>[2x]MAIEIVERSNYMGNPWTEYMAKYDIEEVHGSGIRVDLGEDAEVAGTQYRLPSGKCPVFGKGIIIENSNTAFLTPVATGNQYLKDGGFAFPPTEPLMSPMTLDEMRHFYKDNKYVKNLDELTLCSRHAGNMIPDNDKNSNYKYPAVYDDKDKKCHILYIAAQENNGPRYCNKDESKRNSMFCFRPAKDISFQNY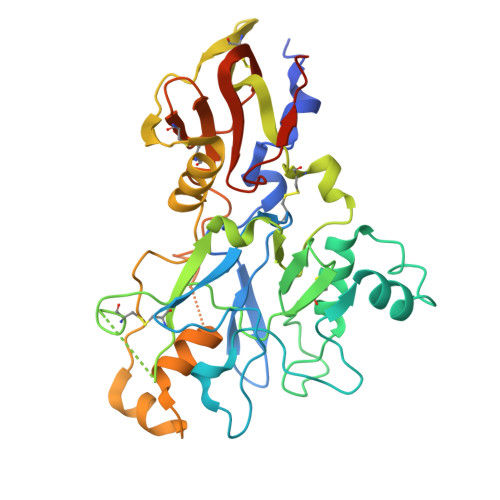AYLSKNVVDNWEKVCPRKNLQNAKFGLWVDGNCEDIPHVNEFPAIDLFECNKLVFELSASDQPKQYEQHLTDYEKIKEGFKNKNAAMIKSAFLPTGAFKADRYKSHGKGYNWGNYNTETQKCEIFNVKPTCLINNAAYIATTALSHPIEVENNFPAAAHHHHHHSEKDEL>[2x]MKEAFKEALARFASGVTVVAARLGEEERGMTATAFMSLSLEPPLVALAVSERAKLLPVLEGAGAFTVSLLREGQEAVSEHFAGRPKEGIALEEGRVKGALAVLRCRLHALYPGGDH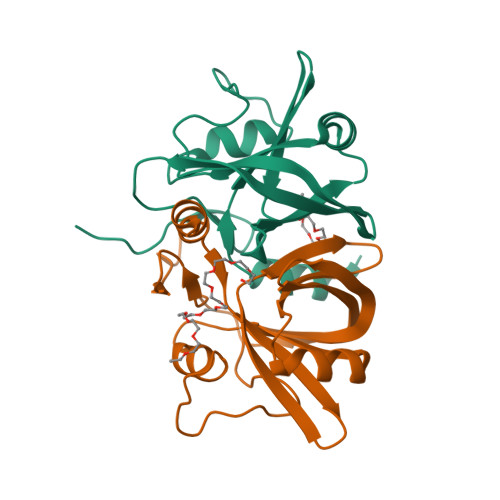RIVVGLVEEVELGEGGPPLVYFQRGYRRLVWPS> EPGLPPGPLENSSAKLVNDEAHPWKPLRPGDIRGPCPGLNTLASHGYLPRNGVATPAQIINAVQEGFNFDNQAAIFATYAAHLVDGNLITDLLSIGRKTRLTGPDPPPPASVGGLNEHGTFEGDASMTRGDAFFGNNHDFNETLFEQLVDYSNRFGGGKYNLTVAGELRFKRIQDSIATNPNFSFVDFRFFTAYGETTFPANLFVDGRRDDGQLDMDAARSFFQFSRMPDDFFRAPSPRSGTGVEVVVQAHPMQPGRNVGKINSYTVDPTSSDFSTPCLMYEKFVNITVKSLYPNPTVQLRKALNTNLDFLFQGVA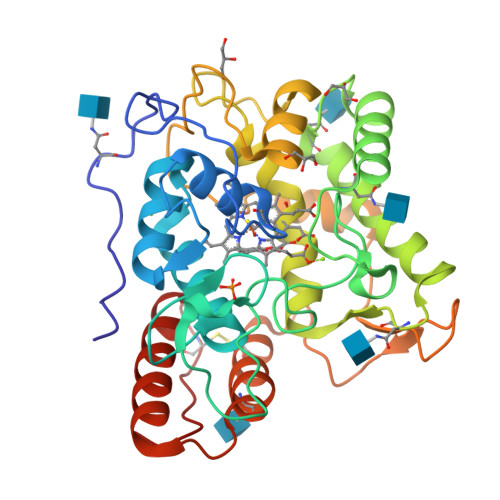AGCTQVFPYGRD>[2x]MKNAPLTLNFGSVRLPVSADGLLHAPTAQQQLGLTQSWEAALVEHGLPE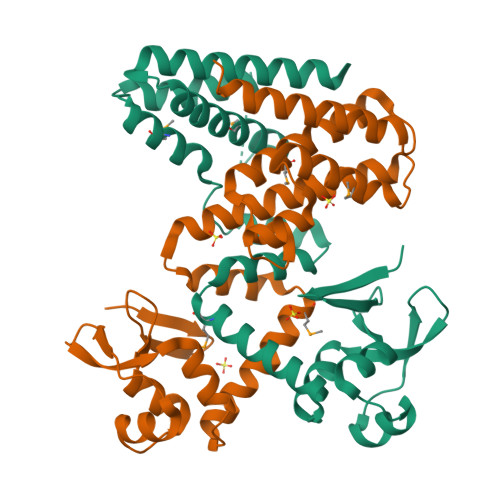TYRDFGAGPEAAVSVPDFVALAFALDTPEARRWQKRARELLARAMQGDVRVAAQIAERNPEPDARRWLAARLESTGARRELMATVARHGGEGRVYGQLGSISNRTVLGKDSASVRQERGVKATRDGLTSAELLRMAYIDTVTARAIQESEARGNAAILTLHEQVARSERQSWERAGQVQRVG Ticks draw blood for days to weeks without eliciting inflammation, and investigation of saliva of the brown dog tick Rhipicephalus sanguineus revealed the presence of chemokine-binding proteins. These proteins, referred to as evasins, suppress chemokine-driven inflammation by binding and neutralizing multiple chemokines. Evasins 1 and 4 (EVA1 and EVA4) are homologous, with eight conserved Cys residues, and specifically bind subsets of CC-chemokines, whereas EVA3 has six Cys residues and specifically binds a subset of ELR+ CXC-chemokines. Members of the first class, which includes the class founder EVA3, bind one or more ELR+ CXC-chemokines, including CXCL1 and/or CXCL8, but not ELR− chemokines.

EVA3 was expressed and purified from Escherichia coli and crystallized readily. The crystal structure of the nonglycosylated EVA3 contains two molecules per asymmetric unit, monomer A (Gly13–Arg66) and monomer B (Asp12–Asn56). The two monomers are very similar, and the Cα of residues 13–56 can be overlaid with a root-mean-square deviation of 1.0 Å. Residues Leu57 to the C-terminal Arg66 are not visible in monomer B and are only visible in monomer A because of an extensive β-sheet interaction of this region of the protein with a symmetry-related monomer. The EVA3 monomer is composed essentially of a single domain containing a large antiparallel β-sheet composed of residues Phe17–Thr27 (β1) and residues Lys47–Gly55 (β3), with residues Phe38–Gly40 forming a third short additional strand (β2) interacting with residues His49–Tyr51 of β3. Two extensive loop regions, composed of residues Ser28–Cys37 and Leu41–Lys47 join the two major β-strands, whereas a very short α-helix is present at the N-terminal region residues Ala14–Asn16. The short β2 strand, which interacts with β3, is held in place by a disulfide bridge between residues Cys26 and Cys39. The first loop, between strands β1 and β2, is rigidified by the presence of two other disulfide bridges between Cys33 and Cys50 and Cys37 and Cys22. The topology of EVA3 is that of an archetypal knottin cystine knot, with the Cys3–Cys6 disulfide bond (Cys33–Cys50 in EVA3) traversing the macrocycle created by Cys1–Cys4 (Cys22–Cys37 in EVA3) and Cys2–Cys5 (Cys26–Cys39 in EVA3) disulfide bonds. The crystal structure also contains a cadmium ion present in the crystallization solution that binds to the side-chain oxygen atoms of Glu60, carbonyl oxygen of Leu57, and carbonyl of Gly36 of the symmetry-related chain A molecule.

>LVSTIESRTSGDGADNFDVVSCNKNCTSGQNECPEGCFCGLLGQNKKGHCYKIIGNLSGEPPVVRR[2x]>[2x]TQPLSKTWELSLYELQRTPQEAITDGLEIVVSPRSLHSELMCPICLDMLKNTMTTKECLHRFCADCIITALRSGNKECPTCRKKLVSKRS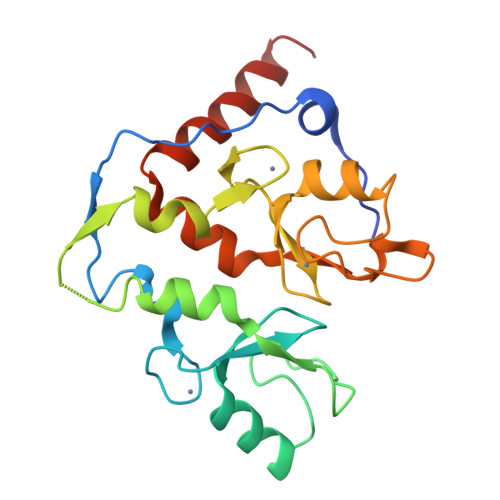LRPDPNFDALISKIYPSMHRTTRIKITELNPHLMCVLCGGYFIDATTIIECLHSFCKTCIVRYLETSKYCPICDVQVHKTRPLLNIRSDKTLQDIVYKLVPGLFKNEMKRRRDFYAAHPSA>GSHMASSAENEIEMRICDYLRRHGRSTVQDIFKELKLEKSTVNRHLYSLQASKQVFKTVEDNKRPVWNLVES[2x]

Unexpectedly, several fish species encode a PKR like kinase in which the two dsRNA-binding domains are substituted by two Z-DNA-binding Zalpha domains. PKZ interacts with CpG repeats, the DNA sequence that is more prone to adopt the left-handed helical conformation of Z-DNA. We expressed and purified the PKZ Zalpha domain (DrZalphaPKZ) encompassing residues 5–70 of zebrafish PKZ (DrPKZ). The protein was crystallized with an oligonucleotide forming a self-complementary (CG)6 DNA duplex with a single T base overhang and resulted in crystals belonging to two different space-groups growing under similar conditions.

The asymmetric unit of the other (hexagonal) crystal form, which belongs to the P6122 space group, contains a single 12 bp-long DNA strand and two DrZalphaPKZ monomers. On the other hand, the hexagonal form shows a 4 bp distance between binding sites with two monomers contacting the central part of the DNA helix and two interacting with the duplex edges. Throughout the article, the hexagonal structure is used as reference, although, if not otherwise stated, descriptions apply to both structures. The Arg62 of the extended wing of monomer B of DrZalphaPKZ forms an additional interaction with the backbone of G6 of the same strand. Interestingly, although the wings of the monomers that face the center of the DNA are well ordered, the wings of the two monomers that face the edge of the duplex are not visible in the electron density, missing residues Glu57-Asn60 and losing the Arg62 contact to DNA. Our structure reveals interactions with the second DNA strand involving Gln27, Phe30 and Lys31, whereas Lys37 is positioned in the middle of the minor groove bridging between the two strands. Also in this case, the monomers positioned at the edge of the DNA are missing these interactions. In our structure, the centrally positioned monomers symmetrically contact each other. The interaction involves the N-terminal edge of α3 of the two monomers and consists of two symmetric salt bridges between Glu36 and Arg42 and hydrogen bonds involving Thr39, Glu36 and Ser38. The guanidinium group of Arg42 is in an interesting arrangement as its Nε also forms a hydrogen bond with the DNA backbone phosphate oxygen.> LRIIWGTNVSIQECTTNFRNFLMSFKYKFRKILDEREEFINNTTDEELYYIKQLNEMRELGTSNLNLDARNLLAYKQTEDLYHQLLNYPQEVISIMDQTIKDCMVSLIVDNNLDYDLDEIETKFYKVRPYNVGSCKGMRELNPNDIDKLINLKGLVLRSTPVIPDMKVAFFKCNVCDHTMAVEIDRGVIQEPARCERIDCNEPNSMSLIHNRCSFADKQVIKLQETPDFVPDGQTPHSISLCVYDELVDSCRAGDRIEVTGTFRSIPIRANSRQRVLKSLYKTYVDVVHVKKVSDKRLDVDTSTIEQELMQNKVDHNEVEEVRQITDQDLAKIREVAAREDLYSLLARSIAPSIYELEDVKKGILLQLFGGTNKTFTKGGRYRGDINILLCGDPSTSKSQILQYVHKITPRGVYTSGKGSSAVGLTAYITRDVDTKQLVLESGALVLSDGGVCCIDEFDKMSDSTRSV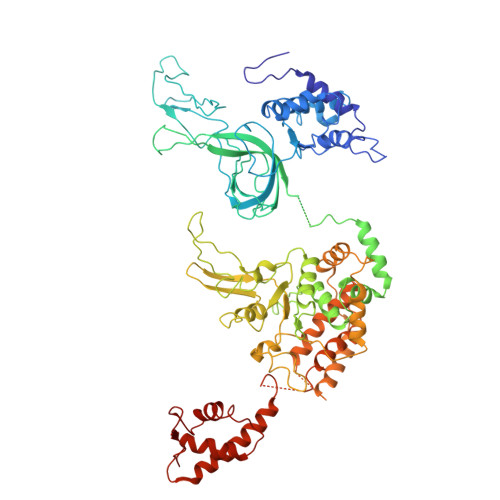LHEVMEQQTISIAKAGIITTLNARSSILASANPIGSRYNPNLPVTENIDLPPPLLSRFDLVYLVLDKVDEKNDRELAKHLTNLYLEDKPEHISQDDVLPVEFLTMYISYAKEHIHPIITEAAKTELVRAYVGMRKMGDDSRSDEKRITATTRQLESMIRLAEAHAKMKLKNVVELEDVQEAVRLIRSAIKDYATDPKTGKIDMNLVQTGKSVIQRKLQEDLSREIMNVLKDQASDSMSFNELIKQINEHSQDRVESSDIQEALSRLQQEDKVIVLGEGVRRSVRL> MSEQSQLDDSTIDKLIPQIFNEMRSNLNNTTNKFPKSTGGGASDNISANSNSIRSFNSITTQSLLKESESLDKITAMIKNVTAALKNNLPVYVNQVHEVCKSTNSILDSWINIHSQAGYIHKLMSDQTYLKLIND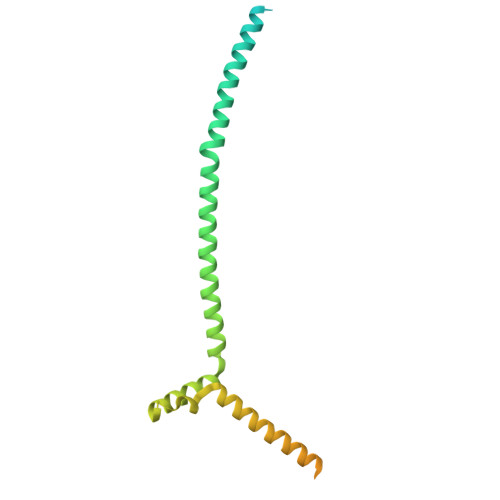RLHNENVNTNDEDGSTLHNVIALKKKEILDLRQKLENRKGEKDAAPAKPPNQGLNPRYGVQSGRRPVPSAGISNNGRVRKTHVPASKRPSGIPRVTNRWTKPTASSSRKMFR> MGSSHHHHHHSQDPNSISTTMSSYSIQQSQKMLTQLQ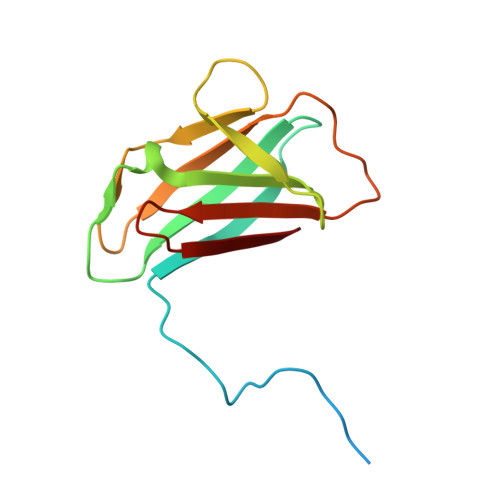IDYATNTSSNTVVAYLHNVGETTISYLQNSVVYFGPNGQLQPVGYNSGSSPYWTVTSNSLQPGSVVKIIIYLSSPLSSNQYYTIQIVTPNGYTVSYMF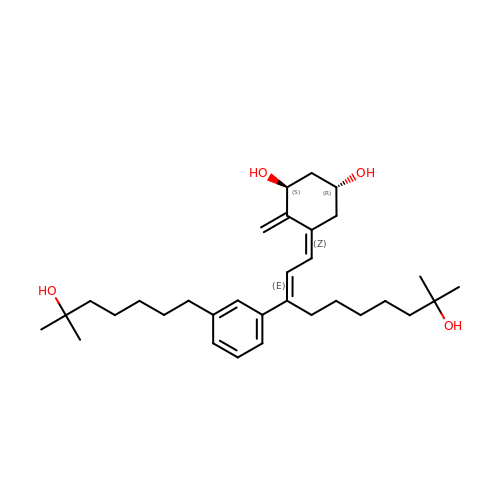(1R,3S,5Z)-4-methylidene-5-[(E)-9-methyl-3-[3-(6-methyl-6-oxidanyl-heptyl)phenyl]-9-oxidanyl-dec-2-enylidene]cyclohexane-1,3-diol | C32 H50 O4 | SQUUCPJJDWEFCT-WWCFBHCMSA-N1-[2-(aminomethyl)phenyl]-N-(3-fluoro-2'-sulfamoylbiphenyl-4-yl)-3-(trifluoromethyl)-1H-pyrazole-5-carboxamide 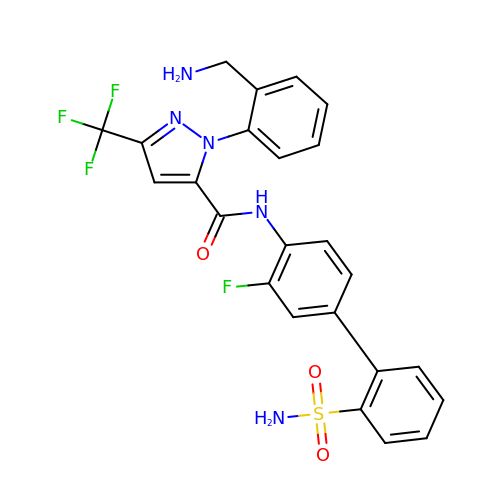| C24 H19 F4 N5 O3 S | TYPXEIGMGZWOGB-UHFFFAOYSA-N>[4x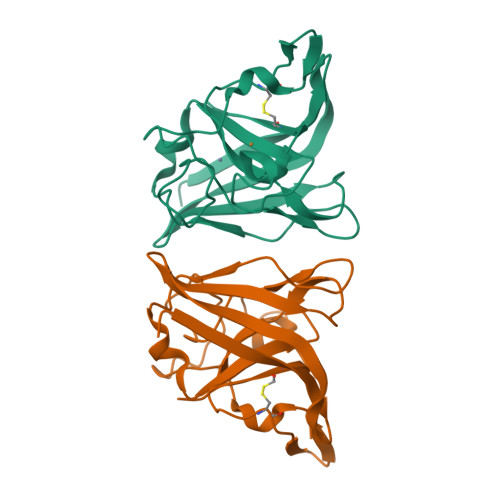]ENTLTVKMNDALSSGTGENIGEITVSETPYGLLFTPHLNGLTPGIHGFHVHTNPSCMPGMKDGKEVPALMAGGHLDPEKTGKHLGPYNDKGHLGDLPGLVVNADGTATYPLLAPRLKSLSELKGHSLMIHKGGDNYSDKPAPLGGGGARFACGVIEKLEHHHHHH3-(4-CARBAMOYL-1-CARBOXY-2-METHYLSULFONYL-BUTA-1,3-DIENYLAMINO)-INDOLIZINE-2-CARBOXYLIC ACID 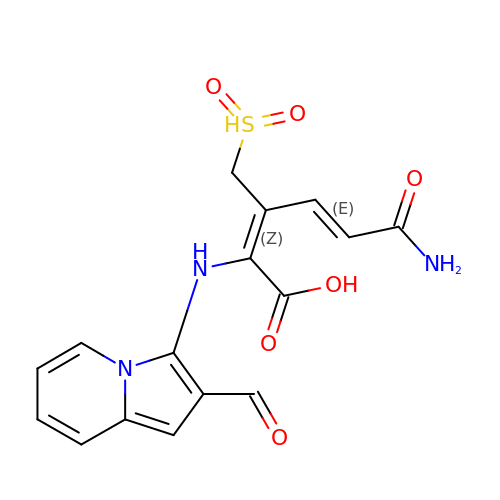| C16 H15 N3 O6 S | ARSFRLAHCNFFCE-IBXIYJDRSA-N>[2x]MTDQAFVTLATNDIYCQGALVLGQSLRRHRLTRKLVVLITPQVSDLLRRILSKVFDEVIEVNLIDSADYIHLAFLKRPELGLTLTKLHCWTLTHYSKCVFLDADTLVLSNVDELFDRGEFSAAPD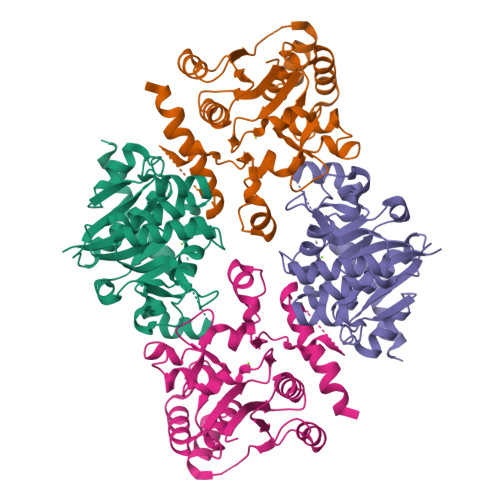PGWPDCFNSGVFVFQPSLHTHKLLLQHAMEHGSFDGADQGLLNSFFRNWSTTDIHKHLPFIYNLSSNTMYTYSPAFKQFGSSAKVVHFLGSMKPWNYKYNPQSGSVLEQGSVSSSQHQAAFLHLWWTVYQNNVLPLYKSVQAENLYFQSHHHHHHDYKDDDDK> MKDHLKQEGKFTYLEKGEGTPI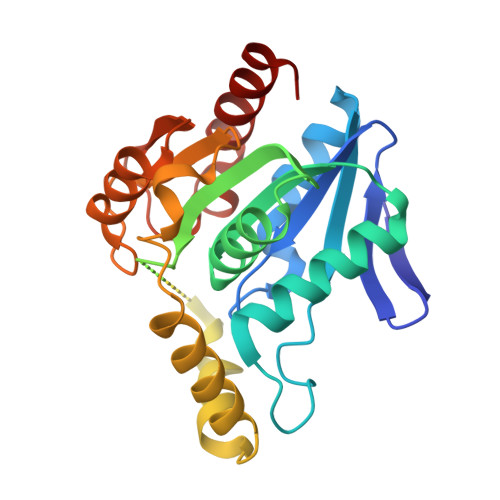VILHGLMGGLSNFDGVIDYFPEKGYKVLIPELPLYSMSLLKTSVGTFARYLKEFVDFKGYENVILLGNSLGGHIALLATKMFPEIVQALVITGSSGLYENAMGESYPRRGDYEFIKKKAEAVFYDPEVATKEIVDEVYETVSDRNKLVKTLAIAKSAIRHNMAKDLPKMKTPTCIIWGKNDNVTPPEVAEDFKRLLPDADLYWIDKCGHAAMMEHPEEFNQLLHEWFKERDF>[4x]MAPKAKIVLVGSGMIGGVMATLIVQKNLGDVVLFDIVKNMPHGKALDTSHTNVMAYSNCKVSGSNTYDDLAGA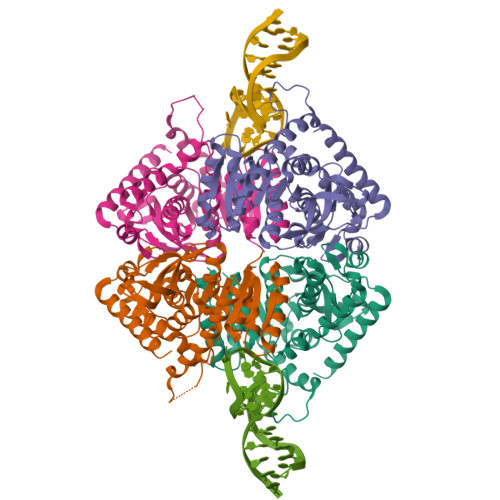DVVIVTAGFTKAPGKSDKEWNRDDLLPLNNKIMIEIGGHIKKNCPNAFIIVVTNPVDVMVQLLHQHSGVPKNKIIGLGGVLDTSRLKYYISQKLNVCPRDVNAHIVGAHGNKMVLLKRYITVGGIPLQEFINNKLISDAELEAIFDRTVNTALEIVNLHASPYVAPAAAIIEMAESYLKDLKKVLICSTLLEGQYGHSDIFGGTPVVLGANGVEQVIELQLNSEEKAKFDEAIAETKRMKALA ethyl 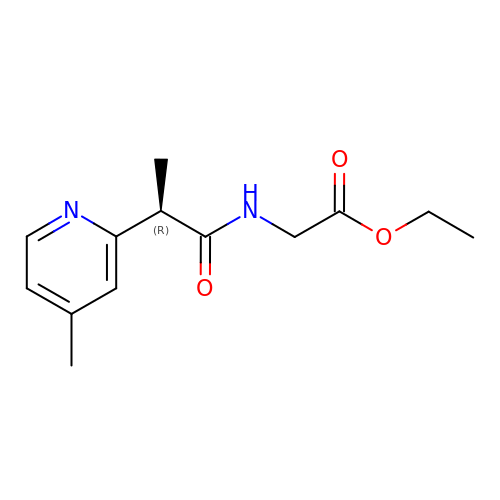N-[(2R)-2-(4-methylpyridin-2-yl)propanoyl]glycinate | C13 H18 N2 O3 | KSDRXGUQEISVKG-SNVBAGLBSA-N> CPPKCRCEKLLFYCDSQGFHSVPNATDKGSLGLSLRHNHITELERDQFASFSQLTWLHLDHNQISTVKEDAFQGLYKLKELILSSNKIFYLPNTTFTQLINLQNLDLSFNQLSSLHPELFYGLRKLQTLHLRSNSLRTIPVRLFWDCRSLEF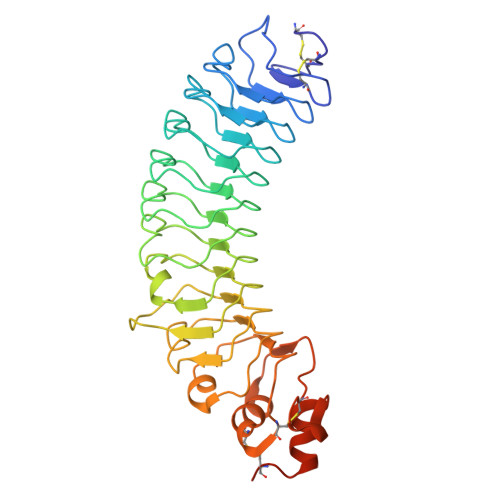LDLSTNRLRSLARNGFAGLIKLRELHLEHNQLTKINFAHFLRLSSLHTLFLQWNKISNLTCGMEWTWGTLEKLDLTGNEIKAIDLTVFETMPNLKILLMDNNKLNSLDSKILNSLRSLTTVGLSGNLWECSARICALASWLGSFQGRWEHSILCHSPDHTQGEDILDAVAGFQLCWNLSTTVTVMAGSHHHHHH>[5x]MHHHHHHGSDDDDKRPEAKSAQPADGWKGERPRSEEDNELNLPNLAAAYSSILSSLGENPQRQGLLKTPWRAASAMQ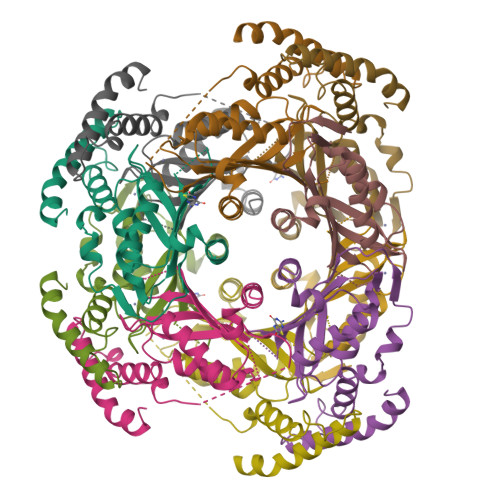FFTKGYQETISDVLNDAIFDEDHDEMVIVKDIDMFSMCEHHLVPFVGKVHIGYLPNKQVLGLSKLARIVEIYSRRLQVQERLTKQIAVAITEALRPAGVGVVVEATHMCMVMRGVQKMNSKTVTSTMLGVFREDPKTREEFLTLIRS>[4x]GALRSLVLIGHGSHHHGESARATQQVAEALRGRGLAGHLPYDEV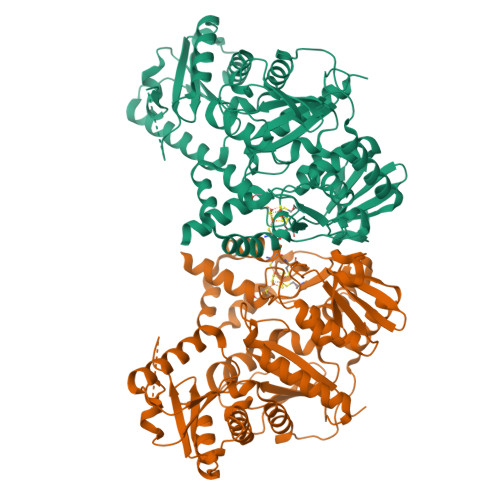LEGYWQQEPGLRQVLRTVAYSDVTVVPVFLSEGYVTETVLPRELGLGHQGPVPTGGVVRVLGGRRVRYTRPLGAHPGMADAIAAQARDTLPEGTDPADVTLLLLAARPGNAALETHAQALRERGQFAGVEVVLESREALTPESHAASAVPLSEWPSRVEAGQAVLVPFLTHLGKHAAERLQQALAQAAERFPQAPPLHVGGPVGEHPAVAEVVLALAAEGREDERGGDIDQAHAEAWAALRHLAERGGRLGEVLLTPYGGLFELRHTLDEGRATLDLQTVVTPEGLRDLTARDEAGRWRPIRTWRTLPRGWRAVLSPADLRLGLELLYPAVIEESYAHEHRRLHWTPWMSTARRQTGTLARVQRATPDQVDTVAAQVCASCLRTRLWAGHTLGQTIFSGVPGGLPCAEACTVLLAAVRDEVGREAMGSGD>MHHHHHHSSGRENLYFQGHVELSSTLLKNLKNFKKENELKKIALTIIAKHLCDVEINNLRNIFIALDVDNSGTLSSQEILDGLKKIGYQKIPPDIHQVLRDIDSNASGQIHYTDFLAATIDKQTYLKKEVCLIPFKFFDIDGNGKISVEELKRIFGRDD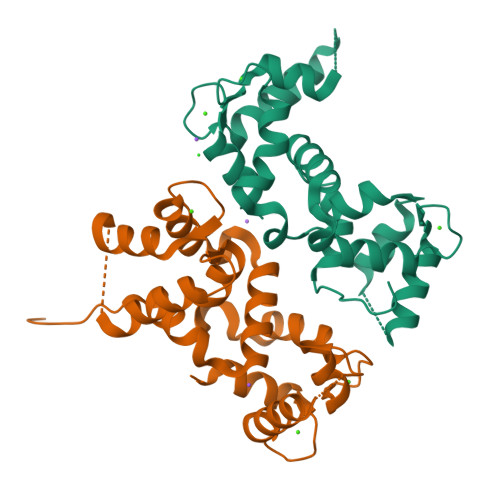IENPLIDKAIDSLLQEVDLNGDGEIDFHEFMLMMSKKK[2x]> AMSAIKPDMRIKLRMEGNVNGHHFVIDGDGTGKPYEGKQTMDLEVKEGGPLPFAFDILTTAFHYGNRVFVKYPDNIQDYFKQSFP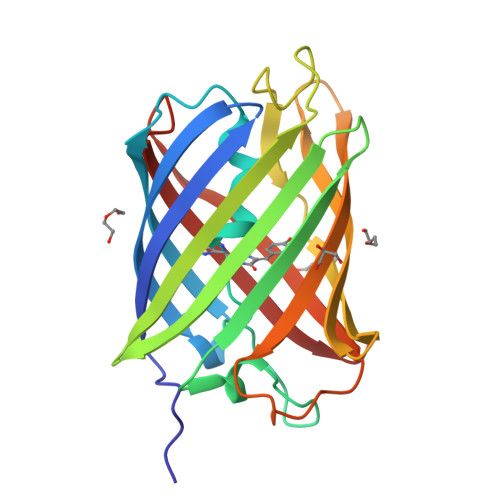KGYSWERSMTFEDGGICNARNDITMEGDTFYNKVRFYGTNFPANGPVMQKKTLKWEPSTEKMYVRDGVLTGDIEMALLLEGNAHYRCDFRTTYKAKEKGVKLPGAHFVDHAIEILSHDKDYNKVKLYEHAVAHSG> MAVNSKYHHSCINCGGLNTDERNERGLPCEVCLPEDSPSDIYRALLERKTLKEYRFYHEFWNEYEDFRSFFKKKFGKDLTGYQRLWAKRIVQGKSFTMVAPTGVGKTTFGMMTALWLARKGKKSALVFPTVTLVKQTLERLQKLADEKVKIFGFYSSMKKEEKEKFEKSFEEDDYHILVFSTQFVSKNREKLSQKRFDFVFVDDVDAVLKASRNIDTLLMMVGIPEEIIRKAFSTIKQGKIYERPKNLKPGILVVSSATAKPRGIRPLLFRDLLNFTVGRLVSVARNITHVRISSRSKEKLVELLEIFRDGILIFAQTEEEGKELYEYLKRFKFNVGETWSEFEKNFEDFKVGKINILIGVQAYYGKLTRGVDLPERIKYVIFWGTPSMRFSLELDKAPRFVLARVLKEMGLIKAQENPDVEELRKIAKEHLTQKEFVEKVKEMFRGVVVKDEDLELIIPDVYTYIQASGRSSRILNGVLVKGVSVIFEEDEEIFESLKTRLLLIAEEEIIEEAEANWKELVHEVEESRRRSERELTDTSRSLLIIVESPTKAETLSRFLGRASSRKERNIIVHEAVTGEGVILFTATRGHVYDLVTKGGIHGVEEENGKFVPVYNSLKRCRDCGYQFTEDRDECPVCSSKNIDDKTETLRALREISLEADEILVATDPDVEGEKISWDVTQYLLPSTRSLRRIEMHEITRYGFKKARESVRFVDFNLVKAQIVRRVQDRWIGFELSGKLQKRFGRSNLSAGRVQSTVLGWIVEREEEYKKSEKDFTLLVLENGVNLEVEGKIADDVVTVVELQEAEEEKNPLPPYTTSSALSEISQKLRLGVQEVMDILQDLFEK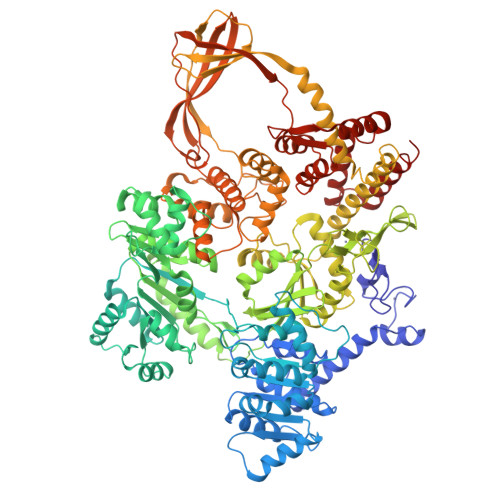GFITYHRTDSTRISLEGQNVARTYLRKIGKEDIFMGRSWSTEGAHEAIRPVKPIDARELEEMIEEGLIADLTKKHLRVYELIFNRFLASQSAAVKVKKQIVTVDVDGKRMGIEQIVEILRDGWNLFVPLTVSPRFEHRTYKIKEKKFYKKHTVPLFTQASIVEEMKKRGIGRPSTYAKIVEVLFRRGYVYEDKYKRVRPTRFGVMVYSYLKERYEKYVTEETTRRLEEIMDKVERGEEDYQATLRLLYEEIKSLMEEG> MAHHHHHHSSGLEVLFQGPDLHVIDHDFLKGQGDARSVRHIAIPAHRGLITDRNGEPLAVSTPVTTLWANPKELMTAKERWPQLAAALGQDTKLFADRIEQNAEREFIYLVRGLTPEQGEGVIALKVPGVYSIEEFRRFYPAGEVVAHAVGFTDVDDRGREGIELAFDEWLAGVPGKRQVLKDRRGRVIKDVQVTKNAKPGKTLALSIDLRLQYLAHRELRNALLENGAKAGSLVIMDVKTGEILAMTNQPTYNPNNRRNLQPAAMRNRAMIDVFEPGSTVKPFSMSAALASGRWKPSDIVDVYPGTLQIGRYTIRDVSRNSRQLDLTGILIKSSNVGISKIAFDIGAESIYSVMQQVGLGQDTGLGFPGERVGNLPNHRKWPKAETATLAYGYGLSVTAIQLAHAYAALANDGKSVPLSMTRVDRVPDGVQVISPEVASTVQGMLQQVVEAQGGVFRAQVPGYHAAGKSGTARKVSVGTKGYRENAYRSLFAGFAPATDPRIAMVVVIDEPSKAGYFGGLVSAPVFSKVMAGALRLMNVPPDNLPTATEQQQVNAAPAKGGRG

Penicillin-binding proteins (PBPs) are membrane-bound enzymes involved in the final stages of bacterial cell wall synthesis on the periplasmic side of the membrane. PBP3 shares 42% sequence identity with the corresponding protein in E. coli and has been identified as the primary target of a number of β-lactams used to treat pseudomonal infections, including the cephalosporin analogues cefsulodin and ceftazidime, piperacillin, and the parenteral carbapenem, doripenem. PBP3 is a two-domain protein comprising a C-terminal transpeptidase linked to an extended N-terminal domain. The active site of PBP3 is located in a long cleft running parallel with the β3 strand across the lower part of the transpeptidase domain.

Three isomorphous structures of P. aeruginosa PBP3 have been determined: apo-PBP3 at 2.0 Å resolution, PBP3/carbenicillin complex at 2.4 Å resolution, and PBP3/ceftazidime complex at 2.6 Å resolution. The SXXK motif (S294-T295-V296-K297) is located at the N-terminal end of α2 and includes the nucleophilic S294, together with the α8–β2f loop (residues 407–409) that forms the base of the cleft. The SXN motif (S349-S350-N351) occurs in the α4–α5 turn, and residues 328–334 (β2c and β2c–β2d loop) form one side of the elongated cleft; the third motif KS/TG (K484-S485-G486) is positioned on strand β3 and, together with residues 530–533 in the β5–α11 loop, forms the opposite side of the cleft. Unlike in PBP2a,12 which is relatively resistant to β-lactam inhibition, the catalytic S294 is positioned favorably for acylation in an open substrate-binding pocket. The three conserved structural motifs interact with each other via a network of hydrogen bonds: the hydroxyl group of S294 forms hydrogen bonds with the side chains of both K297 and K484 (2.7 Å and 2.8 Å), which are hydrogen bonded to S349 and N351, respectively. The position of K297 makes it one of the possible proton receptors from the catalytic S294 during the acylation reaction, in addition to the possible contribution of the β-lactam carboxylate. There are eight water molecules in the active site cleft of apo-PBP3, which form an extensive hydrogen-bonding network with the protein. The two loops connecting β3 and β4 (K490-A500) and β5 and α11 (S526-F531) are disordered in the apo-enzyme.> MVAGHASGSPAFGTASHSNCEHEEIHLAGSIQPHGALLVVSEHDHRVIQASANAAEFLNLGSVLGVPLAEIDGDLLIKILPHLDPTAEGMPVAVRCRIGNPSTEYCGLMHRPPEGGLIIELERAG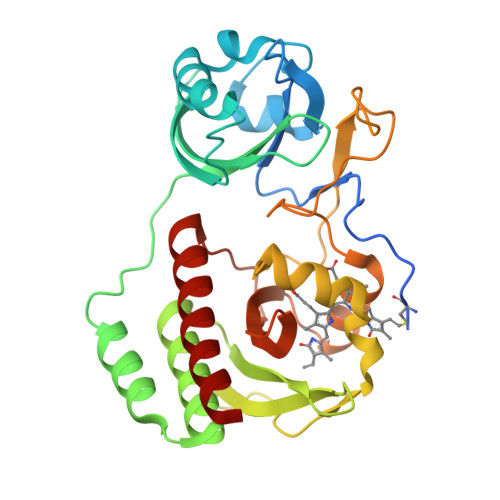PSIDLSGTLAPALERIRTAGSLRALCDDTVLLFQQCTGYDRVMVYRFDEQGHGLVFSECHVPGLESYFGNRYPSSFIPQMARQLYVRQRVRVLVDVTYQPVPLEPRLSPLTGRDLDMSGCFLRSMSPIHLQFLKDMGVRATLAVSLVVGGKLWGLVVCHHYLPRFIRFELRAICKRLAERIATRITALES>MSENQEQEEVITVRVQDPRVQNEGSWNSYVDYKIFLHTNSKAFTAKTSCVRRRYREFVWLRKQLQRNAGLVPVPELPGKSTFFGTSDEFIEKRRQGLQHFLEKVLQSVVLLSDSQLHLFLQSQL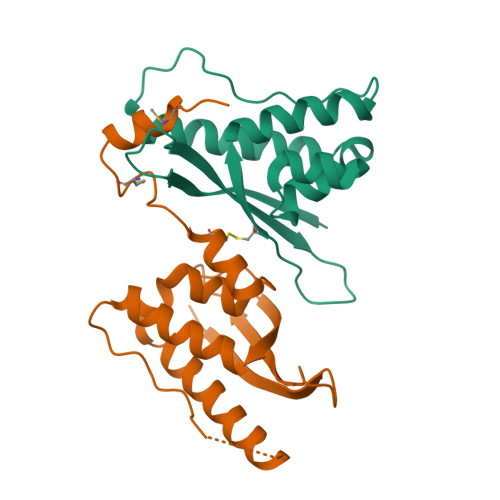SVPEIEACVQGRSTMTVSDAILRYAMSNLEHHHHHH[24x]(3R,4S,7Z)-7-(2-amino-1,3-thiazol-4-yl)-4-formyl-1-[({3-[(5R)-5-hydroxy-4-oxo-4,5-dihydropyridin-2-yl]-4-[3-(methylsulfonyl)propyl]-5-oxo-4,5-dihydro-1H-1,2,4-triazol-1-yl}sulfonyl)amino]-10,10-dimethyl-1,6-dioxo-3-(prop-2-en-1-yl)-9-oxa-2,5,8-triazaundec-7-en-11-oic 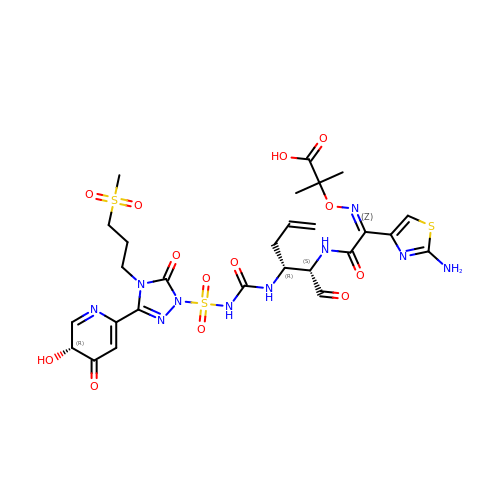acid | C27 H34 N10 O13 S3 | OUKPZOUCAJUMPQ-GDFFEWBWSA-N Brachyury is a transcription factor that plays an essential role in tumour growth of the rare bone cancer chordoma and is implicated in other solid tumours. Brachyury (encoded by the TBXT gene, also formerly known as T) is the founding member of the family and was first identified in 19275. The DNA binding domain forms an immunoglobulin-like fold and contacts DNA via an unusual insertion of an α-helix into the minor groove. All T-box proteins recognize a common consensus sequence named the T-box binding element (AGGTGTGAAA) with family member-specific variations found in the preferences for repeats, orientations (inverted or tandem), and spacing of such repeats.

The chordoma-associated G177D variant brachyury was crystallized with a 26-base pair DNA sequence and diffracted to 2.15 Å resolution. As would be expected with only a single substitution, the structures of the WT and G177D variant are very similar (RMSD 0.8 Å) with only minor differences seen in the ordering and conformations of various loops that are presumably flexible. The G177D substitution itself lies in a loop between strands F and G and is situated away from the DNA interface on the opposite side of the protein. The conformation of this loop is significantly altered with a new salt bridge formed between the substituted D177 residue and R174, possibly explaining the altered conformation in the variant structure. Furthermore, the G177D substitution is within a GGP peptide sequence that lies in a restricted region of Ramachandran space. The PHI and PSI angles adopted by the glycine are not permitted for a non-glycine residue, particularly in the case of a pre-proline which is more restrictive due to steric hindrance around the proline Cδ. The crystallographic B factors indicate this loop is fairly mobile in both the WT and G177D brachyury structures with B factors slightly higher than neighboring residues for both structures, although the potential stabilizing influence of crystal contacts cannot be ruled out. The G177D substitution is however close to the site of the small protein interface that is created between subunits when binding on DNA containing T-box binding sites in a palindromic arrangement. Thus, it is plausible that the substitution may affect the cooperativity of DNA binding as has been suggested previously. Analysis of the interfaces between subunits using the program PISA22 reveals some very minor differences in the interface areas (210 Å2 for the G177D versus 219 Å2 for the WT) and in the calculated energetic contributions towards toward complex formation (−4.8 Kcal/mol versus −4.5 Kcal/Mol); we consider these differences to be unlikely to have a role in the biological activity of brachyury.

>MGELRVGLEESELWLRFKELTNEMIVTKNGRRMFPVLKVNVSGLDPNAMYSFLLDFVAADNHRWKYVNGEWVPGGKPEPQAPSCVYIHPDSPNFGAHWMKAPVSFSKVKLTNKLNGGGQIMLNSLHKYEPRIHIVRVGDPQRMITSHCFPETQFIAVTAYQNEEITALKIKYNPFAKAFLDAKERSHHHHHH[2x]> KTWELSLYELQR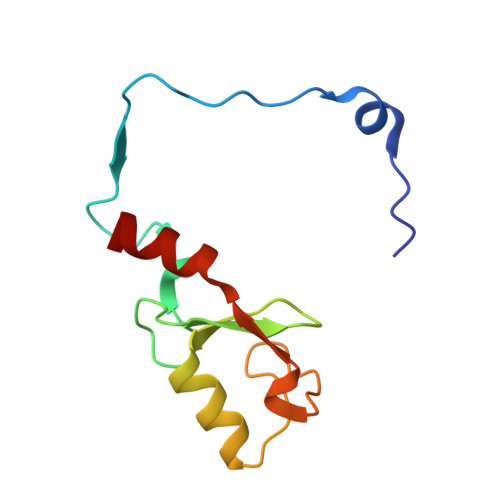TPQEAITDGLEIVVSPRSLHSELMCPICLDMLKNTMTTKECLHRFCADCIITALRSGNKECPTCRKKLVSKRSLRPDPNFDALISKIY> MTTYGSSVPEQQITAYLSRIQRGGYIQPFGCMIAVDESSFRIIGYSENAREMLGIMPQSVPTLEKPEILAMGTDVRSLFTSSSSILLERAFVAREITLLNPVWIHSKNTGKPFYAILHRIDVGVVIDLEPARTEDPALSIAGAVQSQKLAVRAISQLQALPGGDIKLLCDTVVESVRDLTGYDRVMVYKFHEDEHGEVVAESKRDDLEPYIGLHYPATDIPQASRFLFKQNRVRMIVDCNATPVLVVQDDRLTQSMCLVGSTLRAPHGCHSQYMANMGSIASLAMAVIINGNEDDGSNVASGRSSMRLWGLVVCHHTSSRCIPFPLRYACEFLMQAFGLQLNMELQLALQMSEKRVLRTQTLLCDMLLRDSPAGIVTQSPSIMDLVKCDGAAFLYHGKYYPLGVAPSXXXXXXXXXXXXXNHADSTGLSTDSLGDAXXXXXXALGDAVCGMA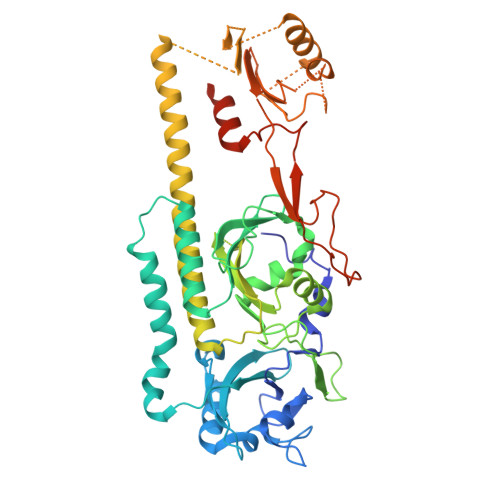VAYITKRDFLFWFRSHTAKEIKWGGAKHHPEDKDDGQRMHPRSSFQAFLEVVKSRSQPWETAEMDAIHSLQLILRDSFKESEAASLHHHHHH> GSHMGGLIYAVGGDGHTHL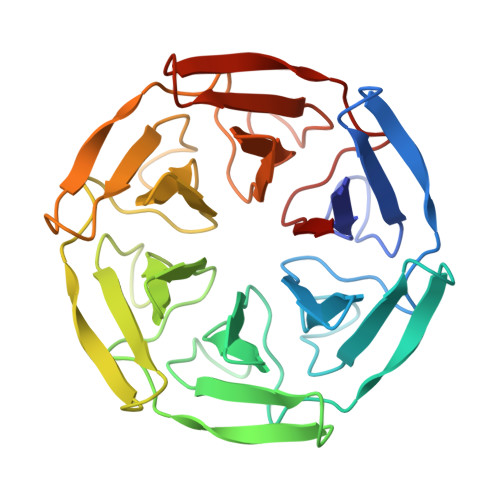SSVEAYNPETNEWSPVAPMSVPRSGVGVAVIGGLIYAVGGDGHTHLSSVEAYNPETNEWSPVAPMSVPRSGVGVAVIGGLIYAVGGDGHTHLSSVEAYNPETNEWSPVAPMSVPRSGVGVAVIGGLIYAVGGDGHTHLSSVEAYNPETNEWSPVAPMSVPRSGVGVAVIGGLIYAVGGDGHTHLSSVEAYNPETNEWSPVAPMSVPRSGVGVAVIGGLIYAVGGDGHTHLSSVEAYNPETNEWSPVAPMSVPRSGVGVAVI> IVGGKVCPKGECPWQVLLLVNGAQLCGGTLINTIWVVSAAHCFDKIKNWRNLIAVLGEHDLSEHDGDEQSRRVAQVIIPSTYVPGTTNHDIALLRLHQPVVLTDHVVPLCLPERTFSERTLAFVRFSLVSGWGQLLDRGATALELMVLNVPRVMTQDCEASYPGKITEYMFCAGYSDGSKDSCKGDSGGPHATHYRGTWYLTGIVSWGQGCATVGHFGVYTRVSQYIEWLQKLMRSEPRPGVLLRAPFP;> ANAFLEELRPGSLERECKEEQCSFEEAREIFKDAERTKLFWISYSDGDQCASSPCQNGGSCKDQLQSYICFCLPAFEGRNCETHKDDQLICVNENGGCEQYCSDHTGTKRSCRCHEGYSLLADGVSCTPTVEYPCGKIPILEK;> SGTTNTVAAYNLTWKSTNFKTILEWEPKPVNQVYTVQISTKSGDWKSKCFYTTDTECDLTDEIVKDVKQTYLARVFSYPAGNVESTGSAGEPLYENSPEFT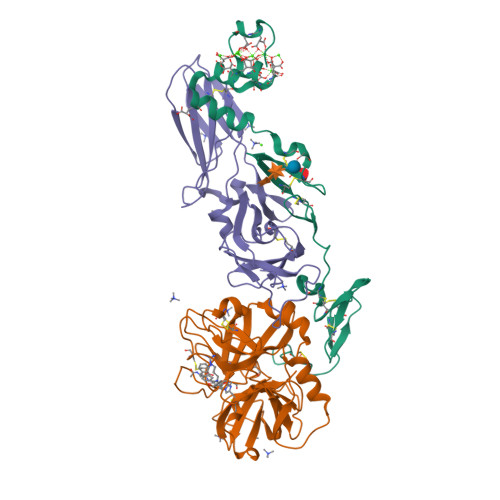PYLETNLGQPTIQSFEQVGTKVNVTVEDERTLVRRNNTFLSLRDVFGKDLIYTLYYWKSSSSGKKTAKTNTNEFLIDVDKGENYCFSVQAVIPSRTVNRKSTDSPVECM> QPSVVEEPGCGPGKVQNGSGNNTRCCSLYAPGKEDCPKERCICVTPEYHCG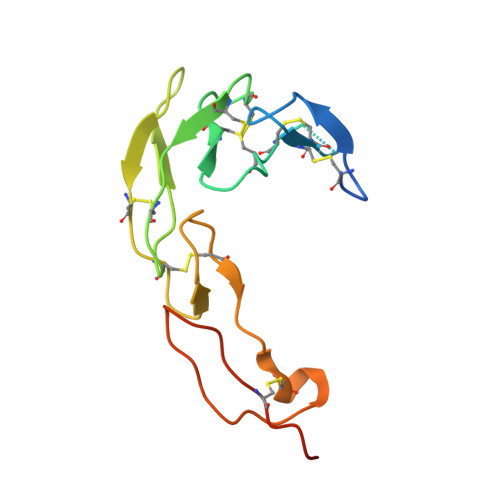DPQCKICKHYPCQPGQRVESQGDIVFGFRCVACAMGTFSAGRDGHCRLWTNCSQFGFLTMFPGNKTHNAVCIPEPLPTEQYGH>[2x]QSNLPEGLDDAYPMTSLQQGMLLQSEASGDPRLLHNVVLHEVHGRLDGELLARAWAILIGRHAILRTGFDLHGGQVPLQWVHPATAVAAEVPVHDLCGLDGETRRLRLRAWIEEEQATPFDWSR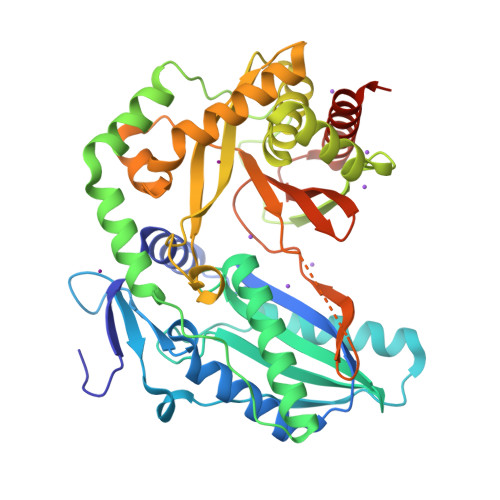PPLVRLAALALDERRFALGVAEHHSVLDGWSLQSLVDELLAVYADLLAGVVAREAEAPAVGFRDYVALEREAEANAASALFWLDYLAGARYRPLPGLAEEGPRRMAAVRVDVPADSLSRLRALAERSGLPLRSLLLAAHGRALCRFSDADEVVTGFVSHGRPEEPGADRLLGLFLNTLPCRLSASVDLLDSARRAFDYERASLEHRRHPLAAIRRRNRELRLDSLFNFVDFHQDDAAPAGVRHGGILDQVVVDVDVPLAVDFEVAGERLEVGFQYAAGRFPAERAEALAGAYREALLALLGDPVQPPAAAQAED> MGSSHHHHHHSQDPGINRKAINFDLSTKSLEKYFKDTREPYSLIKKFMLENGFEHRQYSGYTSKEPINERRVIRIINKLTKKFT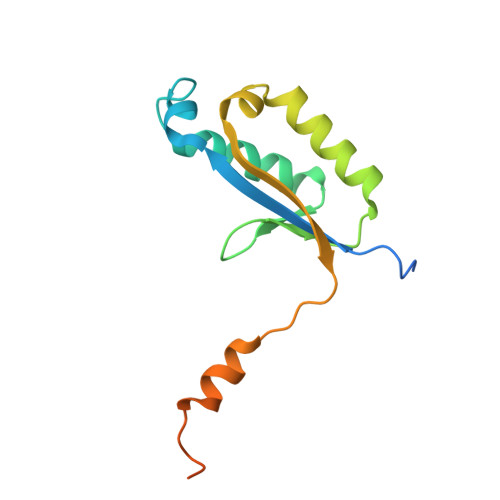WLGECVKEFDITEIGEQYSLKETIQDLCAKDFHQKLKEFTEKTPKNQKLKDLER>[6x]MAVEEI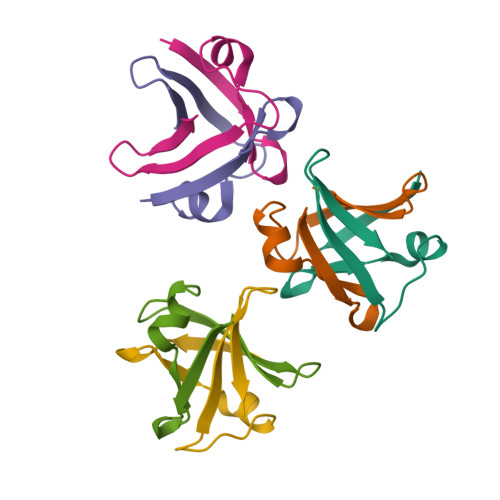VKVSRNYQVTIPAKVRQKFQIKEGDLVKVTFDESEGVVKIQL>APQLHHHHHHDLYENLYFQGKLTTLDEADEAGKRIFGPRVGNELCEVKHVLDLCRIRESVSEELLQLEAKRQELNSEIAKLNLKIEACKKSIENAKQDLLQLKNVISQTEHSYKELMAQNQPKLSLPIRLLPEKDDAGLPPPKATRGCRLHNCFDYSRCPLTSGFPVYVYDSDQFVFGSYLDPLVKQAFQATARANVYVTENADIACLYVILVGEMQEPVVLRPAELEKQLYSLPHWRTDGHNHVIINLSRKSDTQNLLYNVSTGRAMVAQSTFYTVQYRPGFDLVVSPLVHAMSEPNFMEIPPQVPVKRKYLFTFQGEKIESLRSSLQEARSFEEEMEGDPPADYDDRIIATLKAVQDSKLDQVLVEFTCKNQPKPSLPTEWALCGEREDRLELLKLSTFALIITPGDPRLVISSGCATRLFEALEVGAVPVVLGEQVQLPYQDMLQWNEAALVVPKPRVTEVHFLLRSLSDSDLLAMRRQGRFLWETYFSTADSIFNTVLAMIRTRIQIPAAPIREEAAAEIPHRSGKAAGTDPNMADNGDLDLGPVETEPPYASPRYLRNFTLTVTDFYRSWNCAPGPFHLFPHTPFDPVLPSEAKFLGSGTGFRPIGGGAGGSGKEFQAALGGNVPREQFTVVMLTYEREEVLMNSLERLNGLPYLNKVVVVWNSPKLPSEDLLWPDIGVPIMVVRTEKNSLNNRFLPWNEIETEAILSIDDDAHLRHDEIMFGFRVWREARDRIVGFPGRYHAWDIPHQSWLYNSNYSCELSMVLTGAAFFHKYYAYLYSYVMPQAIRDMVDEYINCEDIAMNFLVSHITRKPPIKVTSRWTFRCPGCPQALSHDDSHFHERHKCINFFVKVYGYMPL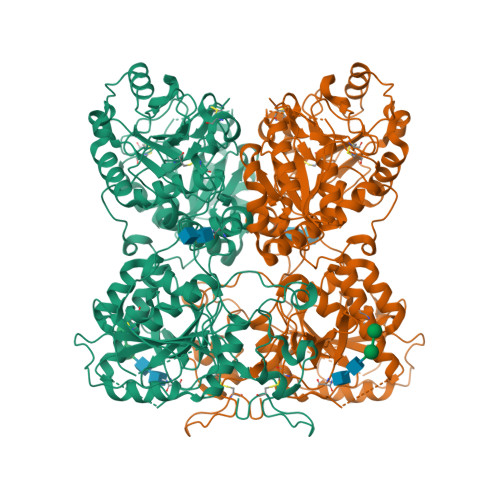LYTQFRVDSVLFKTRLPHDKTKCFKFI[2x]>QAMKELSKSDRTRQFIIESTAPVFNVKGLAGTSLTDLTEATNLTKGSIYGNFENKEAVAIAAFDYNWGHVKSVLTAKVQACNTYKEMLLVYSSMYNDADGSLFPVGGCPLLNTTIEADDTHDALRKKAGEAILSWKKNLVTIIKKGIQAKEFRPDTDVTKIAFSMIALVEGAILIHRATKNRAYSDY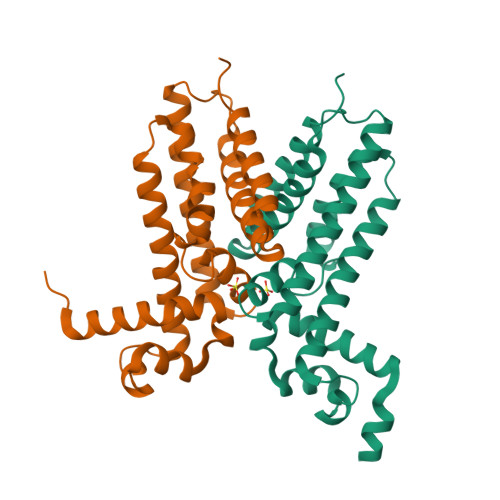VFESLEDLIAGIEVKKK[2x]> GESKSRKRAAPGDNWLPPGWRVEDKIRTSGATAGSVDKYYYEPNTGRKFRSRTEVLYYLEHGTSKRG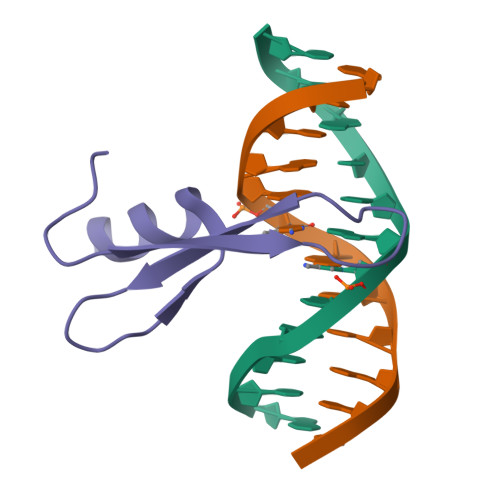TKKAE>GASAPMVKIYTKNGDKGQTRIIGKQILYKNDPRVAAYGEVDELNSWVGYTKSLINSHTQVLSNELEEIQQLLFDCGHDLATPADDERHSFKFKQEQPTVWLEEKIDNYTQVVPAVKKFILPGGTQLASALHVARTITKRAERQIVQLMREEQINQDVLIFINRLSDYFFAAARYANYLEQQPDMLYRNSKDV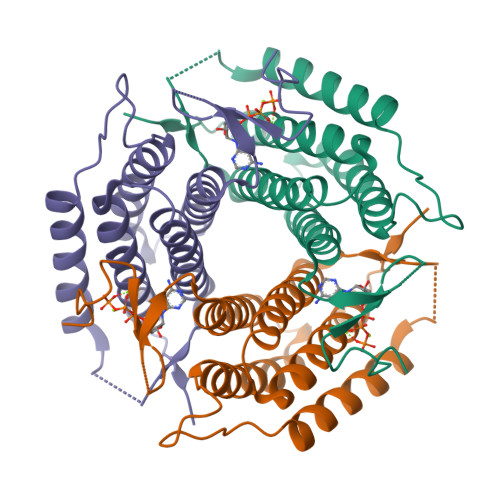FR[2x]> EPLCAVCGQAHSLEENHFYSYPEEVDDDLICHICLQALLDPLDTPCGHTYCTLCLTNFLVEKDFCPMDRKPLVLQHCKKSSILVNKLLNKLLVTCPFREHCTQVLQRCDLEHH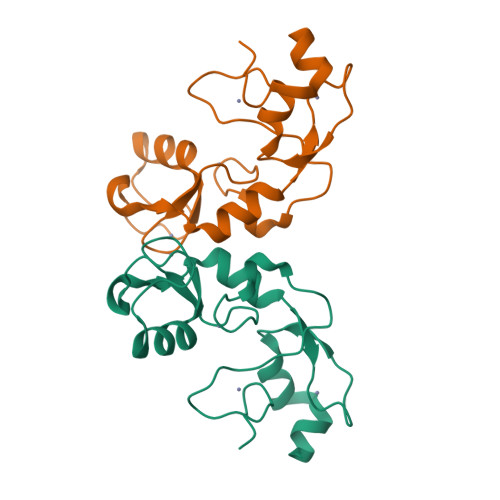FQTSCKGASHYGLTK> MEDASRGEEENSMFETSHVLGALLASSPLLARAWDRCAAAADGGASSLGFVHGGGGGGEGEPVCVAFSGVQAALSAAAGGGGGAEIF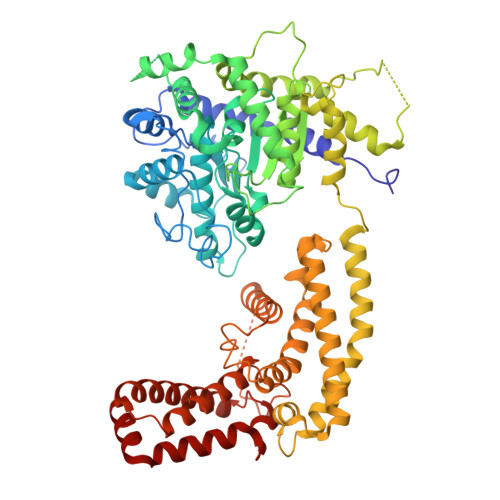KPVGLRGDAAGRLFAPLVAAEPEDAGGEPVAVQALALQGFLRLCRSPEFQVLLNQIRGKAVVFTGHSLGGAIAALVALHYLCTSSSSSAFAPAPPVLCVTFGSPLLGNQALSRAILRERWAGNFCHVVSQHDVVPRLLFCPLNVIPVHIVVGMQLHQLPVRARRAAGVVATVTARMADTNQESLRQLIQEHAGEAAIEQKLAAPEIPSGSPYRPFGAYVLCSPDGAACVDNPTAAVQMLYATFAARRAPETGAVPPEAAHSCYGDLVLSMPHHLLLKRRLGATVTAPAASNYDVGISIALEASGITGEATEAAPARQWLKTSKRVGRSPSLNCASLATRLGRITPCRAQIEWYKALFDANTGYYDAFKQRLSPKKFSKANMYRIKLAQFWDGVLSMLDTSQLPYDFHRRAKWVNAAHFYQLLVEPLDIADYHRNNLHRTRGSYITHGRERRYELFDKWWKQKGCTDPSTGDTSATTTARRSKFAGLTQDPCFWARVEEAREQTESAKSERDMTSLARMLEDLHKFERHSSELVENKEVSIDVVAPQSSYSLWVKEWNELKLREEVRTILFQF> SLLTEVETYVLSIIPSGPLKAEIAQRLEDVFAGKNTDLEVLMEWLKTRPILSPLTKGILGFVFTLTVPSERGLQ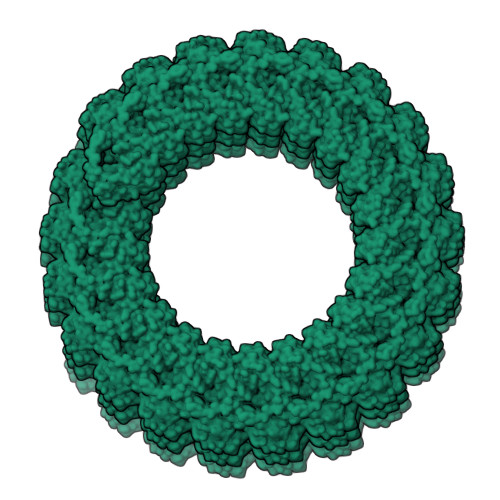RRRFVQNALNGNGDPNNMDKAKKLYRKLKREITFHGAKEISLSYSAGALASCMGLIYNRMGAVTTEVAFGLVCATCEQIADSQHRSHRQMVTTTNPLIRHENRMVLASTTAKAMEQMAGSSEQAAEAMEVASQARQMVQAMRTIGTHPSSSAGLKNDLLENLQAYQKRMGVQMQRFK>MGKDSFTPLYDGGDSSHVHLNKFGSNQLSQSKKSWIARNFSRRECIRFVPKSHDVSRCKCGRPRERHSQQALESGQGSEEWNVASCTTKHPTNAYGEIDFEGYGGQKRAPYLRMSHDTDANLVITLMLKRWNLEIPNLVISVTGGAKSFVLKPRLREMFRRGLIKAAKTTGAWIITGGTNTGVMKHVGEAVKEQQLMFGSDTQVNVIGIATWGIVDKQSDLISEKNGKYPALYSMEPTPGHQGAMLDPNHSHFFLVDDGTEGKYGVEIGMRSRIEEAIMKVKTDSRSEAGSIGVPVVLLVLEGGPNTVATMYELIKKKVPAVVIDGSGRAASVVGFAYNHTIKRNVDGQTINVIDPQYEDEVRAKVVEVFGAKGADKTYSMIKDVLEDEKMISVYSLDGEISQDIDLAILKALLKANRSSPVAQLNLALAWNRIDLAKSDIFTEEQQWTTETLSAAMLTALLDDKAEFAELFLQNGL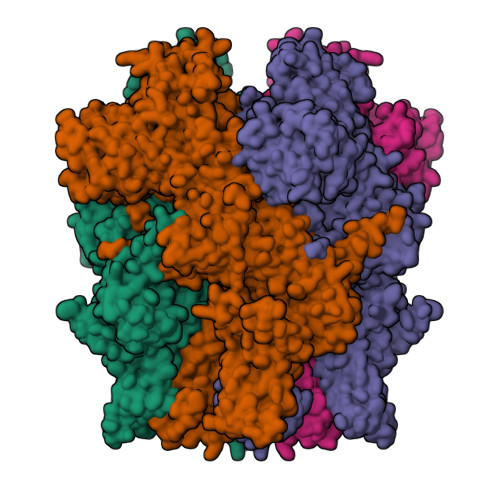SMREFLSLDILCKLYAEVPGNTTIKPLLQKEMGKRQVKTIDMDVVGEVIEELMGDMFESYYRKDGHYFGELASYAEGLVLKNRKSSKDLLANINRIDPLPTPYLDVFLWAVLCNRRELARVLWEAGREPMAAALMASRLLKRMASRAQEDNTITDISSDLYDHARLFEERAVGVLDECFNENETLSQTLLVRELDHYSRMTALELAVSAESQDFIAHTSCQVLLTRLWMGTMAMNTRWWKVLVCLYLPVLIFPIIYFVPDEQHERQAAEREHQKSLNQKSSKVKSHKEKNDAPVVPVYRSKEEKAVSNDEEARVGTENEEEDFQLEDYIPEIREDDSMEVIMRNKKLGFCDRIMHFYSAPFSKFVGNVVGYLAFIFLYAYVVLFNFPRFDPAKTLGGIHPTEIVLYFWVFTILIEEIRQLAAKPPKYIKDKVSVYFSDTWNFVDIFSLTVFIIAIILRFFTNSRIFTASRIILSLDIIFFIVRSLQIFSVNRLLGPKLVMIQKMMQDLAQFIIILAVFTIAYGIALHAVMFPSPGIYARNNTWVTITSVVQYPYWQMYGELFLDEIQGEKPKEFGEVDPDGRWLSPLLLAIYMVFTNILLLNLLIAIFNYTFERVQEDSDKVWKFQRYDLVQEYHSRPVFAPPLVLLGHILIFIRWVWRMCRCGHPPRGSTMKIGLSPAEMEQMDNWEFQAAEMYIHQQQQKNSGTLEERVRALGDRVDCINSQLNRVLDSMSGTRAHALTDGNGLEGGHDSEGRLARMEVELSSNSESLQKILALLQQQPPVKGQAAVPIQLTLLHYKARSSPYPGSTAKRFAVQDNMVDWQVPFPDYKPVNYTAPVVLANPVWADKDLMAMSPRPELPYNQMDHTCNVNRVSYNGTYVVKDGLPLNPMGRTGMQGRGLLGRFGPNHAADPVVTRWKRTSAGVMLQGGKKVLEFVAIQRKDNNQWAIPGGMVEPGQLVTQALKAEFGEEAMAKLNVSQEEKERIAKQIERLFQQGQEIYKGYVDDPRNTDNAWMETVAVNFHDDKGDLFGDITLQAGDDAAAVRWQRVSGNIPLYASHVSILEKVAKMRDAAFSNSLEVLFQ[4x]> MQDAITSVINSSDVQGKYLDSSAIEKLKGYFQTGELRVRAATTIAANAANIIKE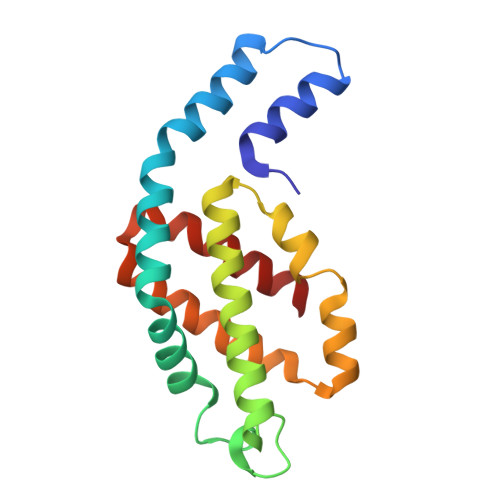AVAKSLLYSDITRPGGNMYTTRRYAACIRDLDYYLRYATYAMLAGDPSILDERVLNGLKETYNSLGVPIGATIQAIQAMKEVTSGLVGPDAGKEMGLYFDYICSGLS> MKLVIEGTIVLKTGM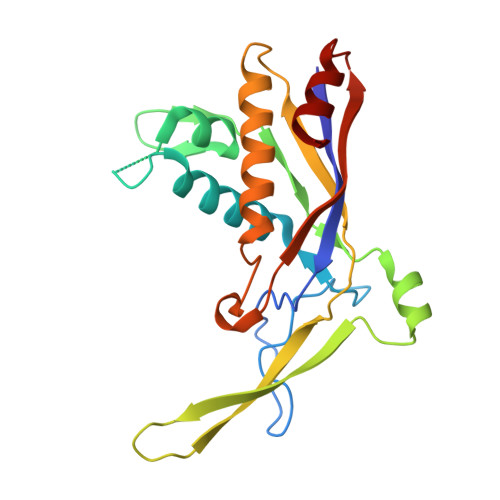HIGGSSDFSAIGAVASPVVRDTLTRLPLIPGSSLKGKMRYLLAKELNNGILLNEPNNDQDEILRLFGSSEKDKIRRARLKFNDIKLSNLAELETFNVSSTEVKFENTINRKTAVANPRQIERVIAGSKFDFEIFYNLDDIKEVEKDFENIKQGFDLLEFDYLGGHGTRGSGRIAFENLSVITAVGNFEKINTLNEILGA3-[(2R)-2-{[(2R)-2-amino-2-phenylacetyl]amino}-2-(dihydroxyboranyl)ethyl]benzoic 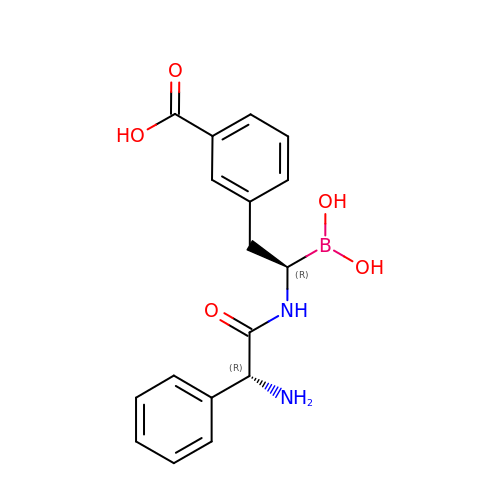acid | C17 H19 B N2 O5 | WMZXFYUXEUIIHA-LSDHHAIUSA-N> MASMTGGQQMGRGSMSILDIAGVDDTLQRLLKEVWFPLRGGEACEKMGYRYDNGVLLHGPSGCGKTTLAHAIAGSIGVAFIPVSAPSVIGGTSGESEKNIRDVFDEAIRLAPCLIFLDQIDAIAGRRESANKGMESRIVAEIMNGMDRIRQNTPLGKNVVVLAATNRPEFLDPAIRRRFSVEIDMGMPSERAREQILRSLTRDLSLADDINFKELAKMTPGYVGSDLQYVVKAAVSESFQANIDSLLAQARAKHPADHLANVSQPQRDWLLLEAHRDEEVSWPSTKITMEQFRKAVSLVQPASKREGFSTIPDTTWSHVGALEDVRKKLEMSIIGPIKNPELFTRVGIKPAAGILLWGPPGCGKTLVAKAVANESKANFISIKGPELLNKYVGESERAVRQLFSRAKSSAPCILFFDQMDALVPRRDDSLSDASARVVNTLLTELDGVGDRSGIYVIGATNRPDMIDEAIRRPGRLGTSIYVGL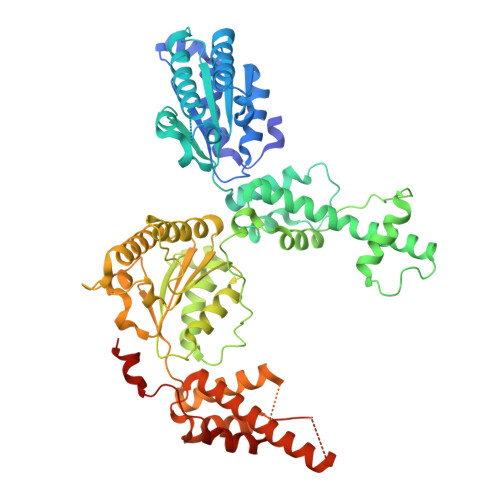PSAEDRVKILKTLYRNTVKAPKKREGTNGEDVDMTDAAAEQQHQGTTDADLEKVALDLRCTGFSGADLGNLMQAAAQACLERVYTQRQQKRKEGGSVAEEEEIEPVITMEDWEKALNEVKPSVKDPEKYMHSGFAAALEHHHHHH> HI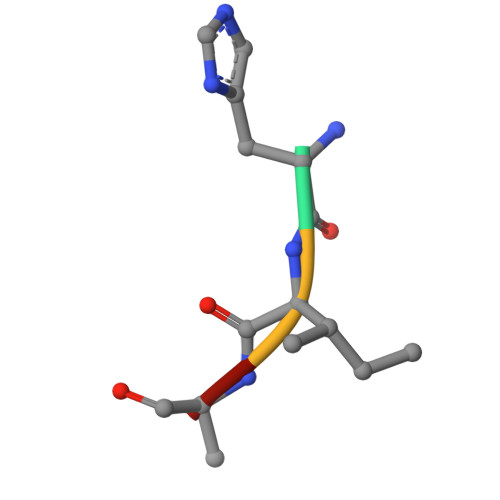AA>[8x]MTKIIKNGTIVTATDTYEAHLLIKDGKIAMIGQNLEEKGAEVIDAKGCYVFPGGIDPHTHLDMPLGGTVTKDDFESGT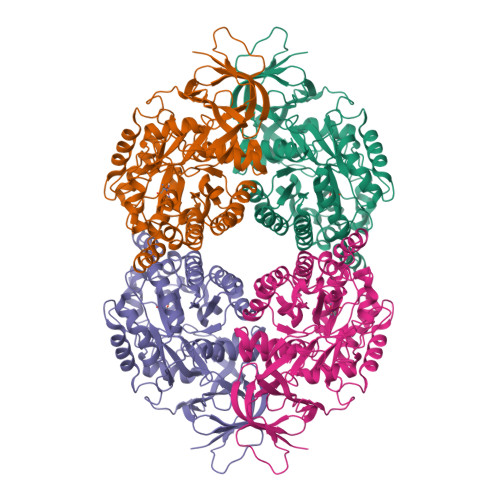IAAAFGGTTTIIDFCLTNKGEPLKKAIETWHNKANGKAVIDYGFHLMISEITDDVLEELPKVLEEEGITSLKVFMAYKNVFQADDGTLYCTLLAAKELGALVMVHAENGDVIDYLTKKALADGNTDPIYHALTRPPELEGEATGRACQLTELAGSQLYVVHVTCAQAVEKIAEARNKGLDVWGETCPQYLVLDQSYLEKPNFEGAKYVWSPPLREKWHQEVLWNALKNGQLQTLGSDQCSFDFKGQKELGRGDFTKIPNGGPIIEDRVSILFSEGVKKGRITLNQFVDIVSTRIAKLFGLFPKKGTIVVGSDADLVIFDPNIERVISAETHHMAVDYNAFEGMKVTGEPVSVLCRGEFVVRDKQFVGKPGYGQYLKRAKYGT>[5x]HTDLSGKVFVFPRESVTDHVNLITPLEKPLQNFTLCFRAYSDLSRAYSLFSYNTQGRDNELLVYKERVGEYSLYI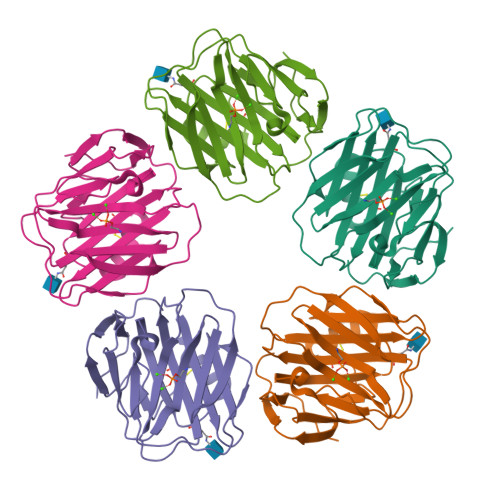GRHKVTSKVIEKFPAPVHICVSWESSSGIAEFWINGTPLVKKGLRQGYFVEAQPKIVLGQEQDSYGGKFDRSQSFVGEIGDLYMWDSVLPPENILSAYQGTPLPANILDWQALNYEIRGYVIIKPLVWV>[2x]KPIEIIGAPFSKGQPRGGVEKGPAALRKAGLVEKLKETEYNVRDHGDLAFVDVPNDSPFQIVKNPRSVGKANEQLAAVVAETQKNGTISVVLGGDESMAIGSISGHARVHPDL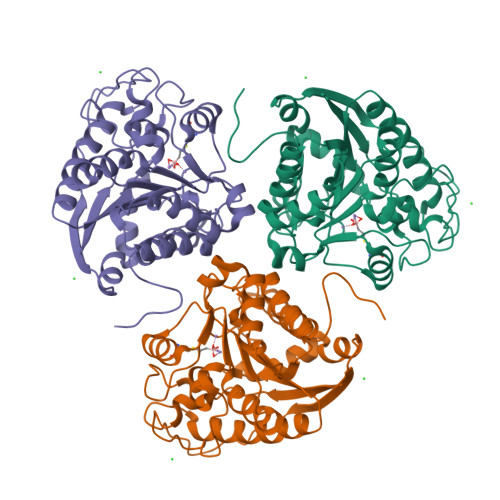CVIWVDAHTDINTPLTTSSGNLHGQPVAFLLKELKGKFPDVPGFSWVTPCISAKDIVYIGLRDVDPGEHYIIKTLGIKYFSMTEVDKLGIGKVMEETFSYLLGRKKRPIHLSFDVDGLDPVFTPATGTPVVGGLSYREGLYITEEIYKTGLLSGLDIMEVNPTLGKTPEEVTRTVNTAVALTLSCFGTKREGNHK(2R,3aR,6S,7aR)-2-[(2S)-2-amino-3-hydroxy-3-oxo-propyl]-6-hydroxy-3,3a,5,6,7,7a-hexahydrofuro[4,5-b]pyran-2-carboxylic 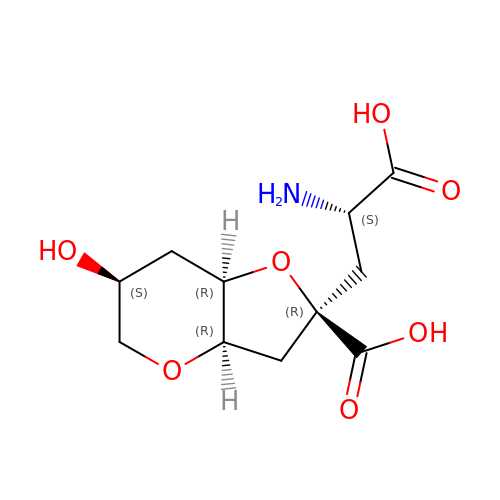acid | C11 H17 N O7 | JVLNPAVKDNEYGY-NRURWVQNSA-N>XS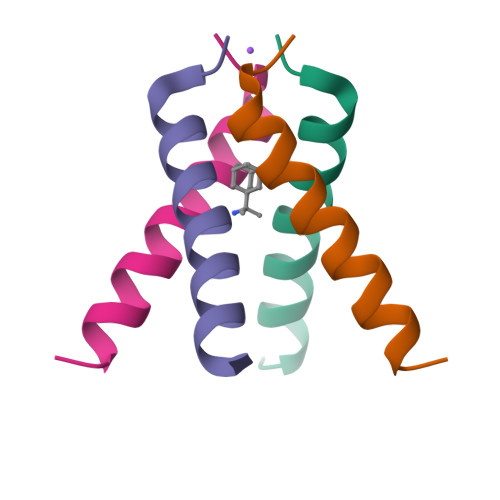SDPLVVAASIIGILHLILWILDRLX[4x]> AIVGVGIDLVSIPDFAEQVDRPGTVFAETFTPGERRDAADKSSSAARHLAARWAA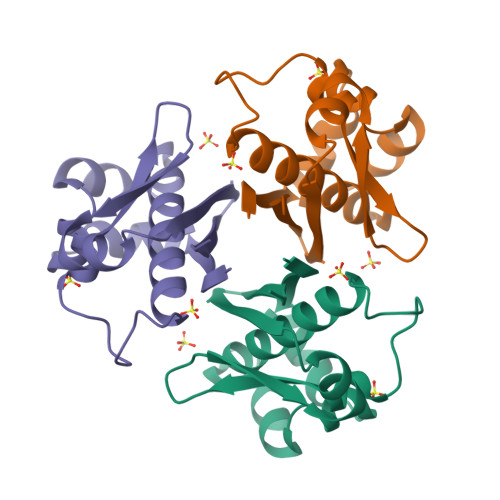KEAVIKAWSSSRFSKRPALPEGIHRDIEVVTDMWGRPKVRLSGEIAKHLEDVTIHVSLTHEDQTAAAVAIIEEP> MKMEARQKQNSFTSKMQKIVNHRAFTFTVIALILFNALIVGIETYPRIYADHKWLFYRIDLVLLWIFTIEIAMRFLASNPKSAFFRSSWNWFDFLIVTLSLVELF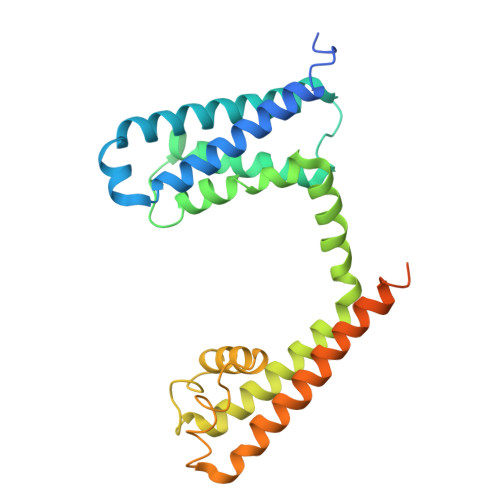LADVEGLSVLRILRVLRVLRAISVVPSLRRLVDALVMTIPALGNILILMSIFFYIFAVIGTMLFQHVSPEYFGNLQLSLLTLFQVVTLESWASGVMRPIFAEVPWSWLYFVSFVLIGTFIIFNLFIGVIVNNVEKAELTDNEEDGEADGLKQEISALRKDVAELKSLLKQSK>[2x]QIGPTETGVV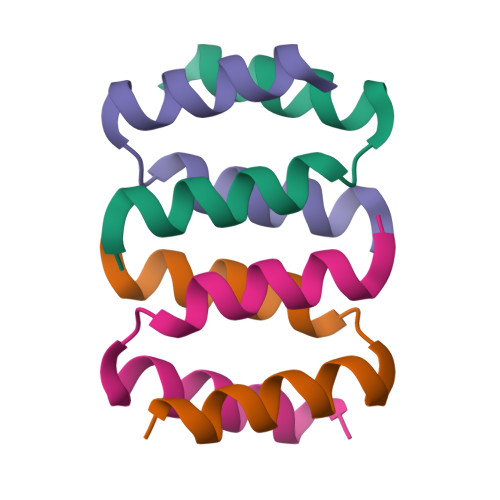QAVKVLLSELSVEGLDEVRRFIDALQ> NYA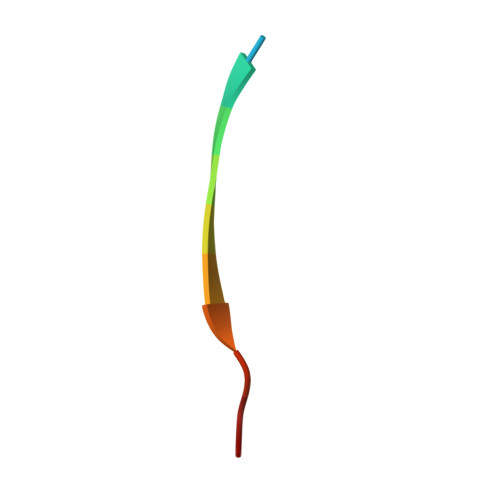ESGIQTDL> TSR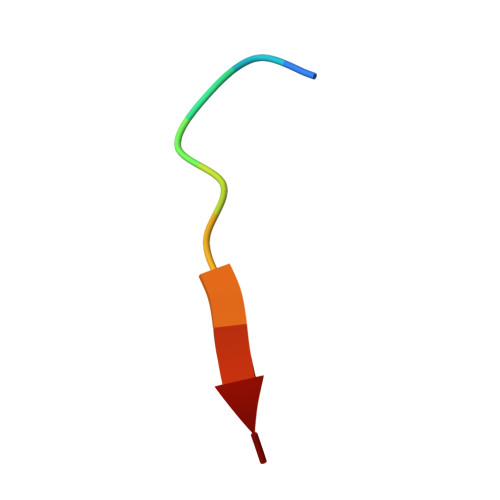QATESTV>MNIMDFNVKKLAADAGTFLSRAVQFTEEKLGQAEKTELDAHLENLLSKAECTKIWTEKIMKQTEVLLQPNPNARIEEFVYEKLDRKAPSRINNPELLGQYMIDAGTEFGPGTAYGNALIKCGETQKRIGTADRELIQTSALNFLTPLRNFIEGDYKTIAKERKLLQNKRLDLDAAKTRLKKAKAAETRNSS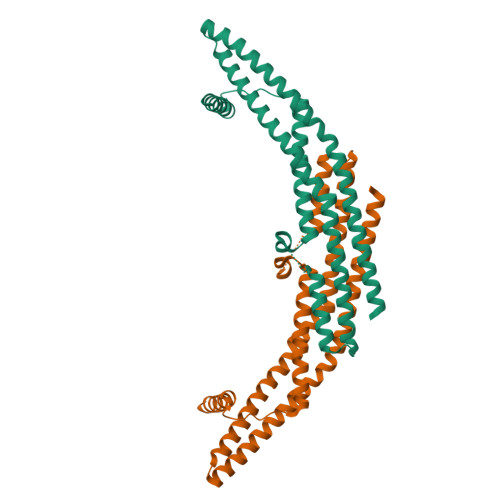EQELRITQSEFDRQAEITRLLLEGISSTHAHHLRCLNDFVEAQMTYYAQCYQYMLDLQKQLGSFPSNYLSNNNQTSVTPVPSVLPNAIGSSAMASTSGLVITSPSNLSDLKECSGSRKARVLYDYDAANSTELSLLADEVITVFSVVGMDSDWLMGERGNQKGKVPITYLELLN[2x]> MVDGNYSVASNVMVPMRDGVRLAVDLYRPDADGPVPVLLVRNPYDKFDVFAWSTQSTNWLEFVRDGYAVVIQDTRGLFASEGEFVPHVDDEADAEDTLSWILEQAWCDGNVGMFGVSYLGVTQWQAAVSGVGGLKAIAPSMASADLYRAPWYGPGGALSVEALLGWSAKIGTGLITSRSDARPEDAADFVQLAAILNDVAGAASVTPLAEQPLLGRLIPWVIDQVVDHPDNDESWQSISLFERLGGLATPALITAGWYDGFVGESLRTFVAVKDNADARLVVGPWSHSNLTGRNADRKFGIAATYPIQ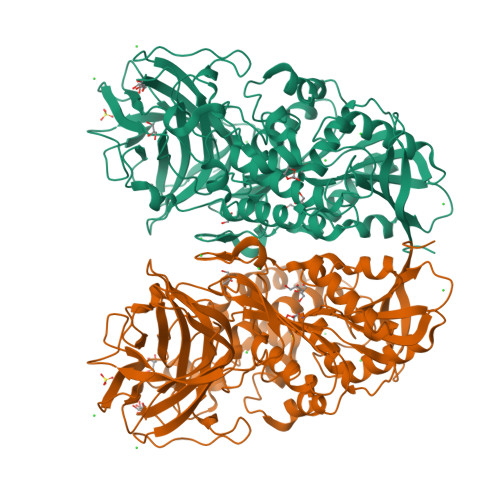EATTMHKAFFDRHLRGETDALAGVPKVRLFVMGIDEWRDETDWPLPDTAYTPFYLGGSGAANTSTGGGTLSTSISGTESADTYLYDPADPVPSLGGTLLFHNGDNGPADQRPIHDRDDVLCYSTEVLTDPVEVTGTVSARLFVSSSAVDTDFTAKLVDVFPDGRAIALCDGIVRMRYRETLVNPTLIEAGEIYEVAIDMLATSNVFLPGHRIMVQVSSSNFPKYDRNSNTGGVIAREQLEEMCTAVNRIHRGPEHPSHIVLPIIKRKLAAALEHHHHHH>[8x]MLKKVED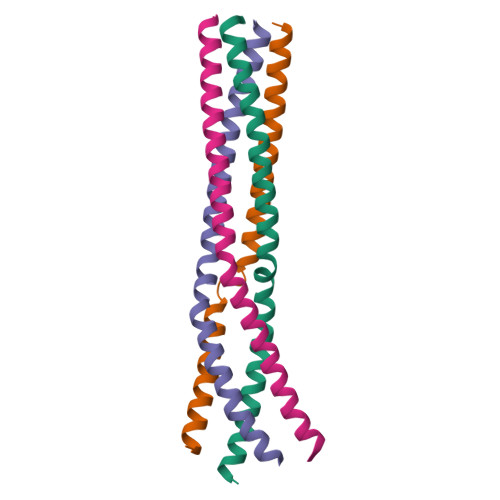TLTMLVNATSRQNAAIEALENRLSTLESSLKPIQDMGKVISSLNRSCAEMVAKYDLLEHHHHHH>MAADAPGDRMEEPLPDRAVPIYVAGFLALYDSGDSGELALDPDTVRAALPPDNPLPINVDHRAGCEVGRVLAVVDDPRGPFFVGLIACVQLERVLETAASAAIFERRGPPLSREERLLYLITNYLPSVSLATKRLGGEAHPDRTLFAHVALCAIGRRLGTIVTYDTGLDAAIAPFRHLSPASREGARRLAAEAEIALSGRTWAPGVEALTHTLLSTAVNNMMLRDRWSLVAERRRQAGIAGHTYLQASEKFKMWGAEPVSAPARGYKNGAPESTDIPPGSIAAAPQGDRCPIVRQRGVALSPVLPPMNPVPTSGTPAPAPPGDGSYLWIPASHYNQLVAGHAAPQPQPHSAFGFPAAAGAVAYGPHGAGLSQHYPPHVAHQYPGVLFSGPSPLEAQIAALVGAIAADRQAGGQPAAGDPGVRGSGKRRRYEAGPSESYCDQDEPDADYPYYPGEARGGPRGVDSRRAARQSPGTNETITALMGAVTSLQQELAHMRARTSAPYGMYTPVAHYRPQVGEPEPTTTHPALCPPEAVYRPPPHSAPYGPPQGPASHAPTPPYAPAACPPGPPPPPCPSTQTRAPLPTEPAFPPAATGSQPEASNAEAGALVNASSAAHVDVDTARAADLFVSQMMGAR[12x];>MTAPRSWAPTTRARGDTEALCSPEDGWVKVHPTPGTMLFREILHGQLGYTEGQGVYNVVRSSEATTRQLQAAIFHALLNATTYRDLEADWLGHVAARGLQPQRLVRRYRNAREADIAGVAERVFDTWRNTLRTTLLDFAHGLVACFAPGGPSGPSSFPKYIDWLTCLGLVPILRKRQEGGVTQGLRAFLKQHPLTRQLATVAEAAERAGPGFFELALAFDSTRVADYDRVYIYYNHRRGDWLVRDPISGQRGECLVLWPPLWTGDRLVFDSPVQRLFPEIVACHSLREHAHVCRLRNTASVKVLLGRKSDSERGVAGAARVVNKVLGEDDETKAGSAASRLVRLIINMKGMRHVGDINDTVRAYLDEAGGHLIDAPAVDGTLPGFGKGGNSRGSAGQDQGGRAPQLRQAFRTAVVNNINGVLEGYINNLFGTIERLRETNAGLATQLQERDRELRRATAGALERQQRAADLAAESVTGGCGSRPAGADLLRADYDIIDVSKSMDDDTYVANSFQHPYIPSYAQDLERLSRLWEHELVRCFKILCHRNNQGQETSISYSSGAIAAFVAPYFESVLRAPRVGAPITGSDVILGEEELWDAVFKKTRLQTYLTDIAALFVADVQHAALPPPPSPVGADFRPGASPRGRSRSRSPGRTAPGAPDQGGGIGHRDGRRDGRR[12x]

Three capsid types have been recognized from the nuclei of herpesvirus-infected cells: empty A-capsids, scaffolding-containing B-capsids, and DNA-filled C-capsids. A unique portal vertex exists at a 12th I5 vertex through which the genome is translocated during assembly. Here, portal proteins assemble into a dodecameric basket-like structure that is thought to seed the assembly of scaffolding proteins, in turn driving the formation of spherical procapsids composed of MCP, SCP, and triplexes. A separate protein complex, the terminase, associates with the dodecameric portal and initiates genome packaging and the concurrent autoproteolytic cleavage of the scaffold.

To improve the resolution of the portal baskets, we carried out separate sub-particle reconstructions and refined them while imposing C12 symmetry, leading to portal basket structures at resolutions of 3.6, 3.5, and 3.7 Å for the A-, B-, and C-capsids, respectively. Additionally, an “anchoring” segment of the scaffold protein is resolved interacting with the portal baskets of A- and B-capsids but not D- and C-capsids. The C12 reconstruction of both A- and B-capsid portal baskets revealed a small hook-like density with large aromatic side chains and sharp turns wedged into a hydrophobic pocket between the crown domains of each portal monomer. This density is weaker in A-capsids, but still conspicuous, whereas it is completely absent in C-capsids, D-capsids, and mature virions (Fig. 4C through E and H through J). Indeed, we found the scaffolding protein residues 449–455 (PYYPGEA, numbered relative to pUL26) to be a good fit for the small density. Based on our model, P452 interacts with the essential residues W127 and L131 (both adjacent to W90) from the first portal monomer, whereas Y451 forms a hydrophobic interface with Y83 and Y608 from the second portal monomer. Furthermore, E454 from the scaffolding appears to stabilize Y608 via hydrogen bonding, buttressing the hydrophobic interactions between the three aromatic residues. Sequence alignment of scaffolding and portal proteins showed that Y608 and Y83 are highly conserved across herpesviruses, suggesting this motif is essential for portal-scaffold association. A- and B-capsids varied in portal height by ~2 and ~1 nm, respectively, could rotate up to 13 degrees relative to the capsid shell, and exhibited up to 1 nm of portal basket “sway,” due to flexibility between the clip and nearby wing and stem domains. In addition to scaffold-capsid interactions, our structure shows high-resolution details of the scaffold-portal interface, enabling the first atomic model of a portion of the scaffolding protein and revealing its tightly packed, hydrophobic nature nestled between portal monomers (G and K through M).>[2x]SMSTKSVLF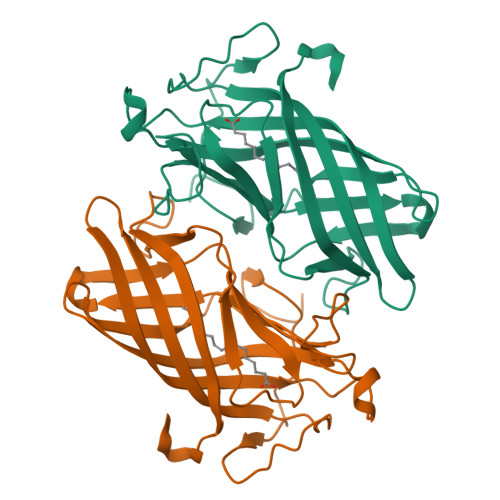GRPVQTEGVPNVYAGAPVVPWTPPEPGIDNLGINSIDTFAVPGVGEYTVAFDGWVRVVRSPSTSGEWADAEVYTNLIEMKMVGECEELGKITVTLNPDCLSAGQIRTPFDPYAGEGPSAKACRMAVGAIFDMPKLGLKLMNREPIILTIDDVRSIPPAGAPGKGQIYRMMPLLDVNDPDGQPVAYLTSLRFNMGGYLKPDQM> VLEEDREPDVIEVNSLEEFDEIMSMDILTVALFWADDCGPCKLIEEPLRKMAEEFPNVVFALVDADKNPEIVKKLNIKSLPTAVIARSGEYLGDV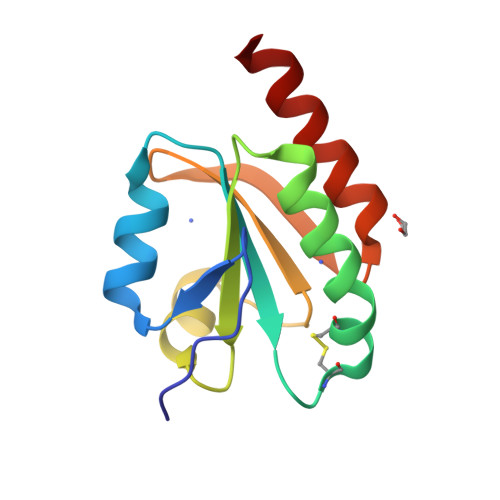VGARPDLLREKVENILKNLE> PISPIETVPVKLKPGMDGP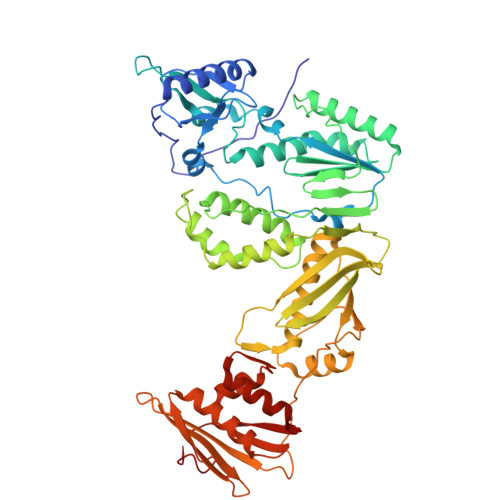KVKQWPLTEEKIKALVEICTEMEKEGKISKIGPENPYNTPVFAIKKKDSTKWRKLVDFRELNKRTQDFWEVQLGIPHPAGLKKKKSVTVLDVGDAYFSVPLDEDFRKYTAFTIPSINNETPGIRYQYNVLPQGWKGSPAIFQSSMTKILEPFAAQNPDIVIYQYMDDLYVGSDLEIGQHRTKIEELRQHLLRWGLTTPDKKHQKEPPFLWMGYELHPDKWTVQPIVLPEKDSWTVNDIQKLVGKLNWASQIYPGIKVRQLSKLLRGTKALTEVIPLTEEAELELAENREILKEPVHGVYYDPSKDLIAEIQKQGQGQWTYQIYQEPFKNLKTGKYARMRGAHTNDVKQLTEAVQKITTESIVIWGKTPKFKLPIQKETWETWWTEYWQATWIPEWEFVNTPPLVKLWYQLEKEPIVGAETFYVDGAANRETKLGKAGYVTNKGRQKVVPLTNTTNQKTELQAIYLALQDSGLEVNIVTDSQYALGIIQAQPDKSESELVNQIIEQLIKKEKVYLAWVPAHKGIGGNEQVD>VGGSDERFLCRSIRKLVYPKKGLRADDTWQLIVNNDEYKQAIQIEECEGADQPCDFAANFPQSYNPICKQHYTQQTLASIKSDGELDVVQN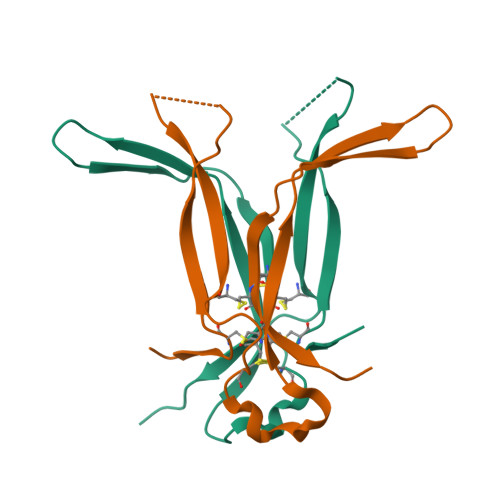SFKIPSCCKCALKTGLEHHHHHH[2x]Human NAD-dependent isocitrate dehydrogenase or IDH3 (HsIDH3) catalyzes the decarboxylation of isocitrate into α-ketoglutarate in the tricarboxylic acid cycle. It consists of three types of subunits (α, β, and γ) and exists and functions as the (αβαγ)2 heterooctamer. HsIDH3 is regulated allosterically and/or competitively by numerous metabolites including CIT, ADP, ATP, and NADH. In this work, we report the crystal structures of the αβ and αγ heterodimers and the (αβαγ)2 heterooctamer containing an α-Q139A mutation in the clasp domain, which renders all the heterodimers and the heterooctamer constitutively active in the absence of activators.

Crystals of αMMgβADP belong to space group I422, and the asymmetry unit contains one αMβ heterodimer, which forms an (αMβ)2 heterotetramer with a crystallographic 2-fold axis-related heterodimer. In this structure, there is an Mg2+ ion bound at the active site in the α subunit and an ADP bound at the pseudo-allosteric site in the β subunit, which are well defined in the electron density map. In the αβ, αMβ, and αMMgβADP structures, the active site assumes an “open” conformation due to the absence of substrate and/or cofactor. Intriguingly, in this study, we found that there is an ADP bound at the pseudo-allosteric site with clearly defined electron density in the αMMgβADP structure, and there is an NAD bound at the pseudo-allosteric site albeit only the ADP-ribose moiety is well defined while the nicotinamide moiety is poor defined in the electron density map in the αMICT+Ca+NADβNAD structure. The binding of ADP/NAD at the pseudo-allosteric site causes substantial conformational changes of the sidechains of His275B and Phe277B, which induce the β12B-α8B loop to adopt a conformation similar to that of the β12G-α8G loop in the WT αγ heterodimer. In the αMMgβADP and αMICT+Ca+NADβNAD structures, ADP or NAD form hydrogen bonds with His275B, Phe277B, Ala278B, and Asn287B (corresponding to Asn273G, Gly275G, Lys276G, and Asn287G) in the β12B-α8B loop and Thr207A from the α small domain. Besides, the sidechain of Phe277B makes a π-π interaction with the adenine moiety of the ligand, which further stabilizes the ligand binding. The ADP binding at the pseudo-allosteric site may in turn stabilize the active conformation of the αβ-αβ interface and the active site, which may explain our biochemical data showing that the addition of activators has a weak activation effect (1.7-fold) for the αMβ heterodimer but not for the WT αβ heterodimer.

> TGGVQTVTLIPGDGIGPEISAAVMKIFDAAKAPIQWEERNVTAIQGPGGKWMIPSEAKESMDKNKMGLKGPLKTPIAAGHPSMNLLLRKTFDLYANVRPCVSIEGYKTPYTDVNIVTIRENTEGEYSGIEHVIVDGVVASIKLITEGASKRIAEFAFEYARNNHRSNVTAVHKANIMRMSDGLFLQKCREVAESCKDIKFNEMYLDTVCLNMVQDPSQFDVLVMPNLYGDILSDLCAGLIGGLGVTPSGNIGANGVAIFESVHGTAPDIAGKDMANPTALLLSAVMMLRHMGLFDHAARIEAACFATIKDGKSLTKDLGGNAKCSDFTEEICRRVKDLD;> ASRSQAEDVRVEGSFPVTMLPGDGVGPELMHAVKEVFKAAAVPVEFQEHHLSEVQNMASEEKLEQVLSSMKENKVAIIGKIHTPMEYKGELASYDMRLRRKLDLFANVVHVKSLPGYMTRHNNLDLVIIREQTEGEYSSLEHESARGVIECLKIVTRAKSQRIAKFAFDYATKKGRGKVTAVHKANIMKLGDGLFLQCCEEVAELYPKIKFETMIIDNCCMQLVQNPYQFDVLVMPNLYGNIIDNLAAGLVGGAGVVPGESYSAEYAVFETGARHPFAQAVGRNIANPTAMLLSASNMLRHLNLEYHSSMIADAVKKVIKVGKVRTSDMGGYATCHDFTEEICRRVKDLDEN> MATVEPETTPTPNPPTTEEEKTESNQEVANPEHYIKHPLQNRWALWFFKNDKSKTWQANLRLISKFDTVEDFWALYNHIQLSSNLMPGCDYSLFKDGI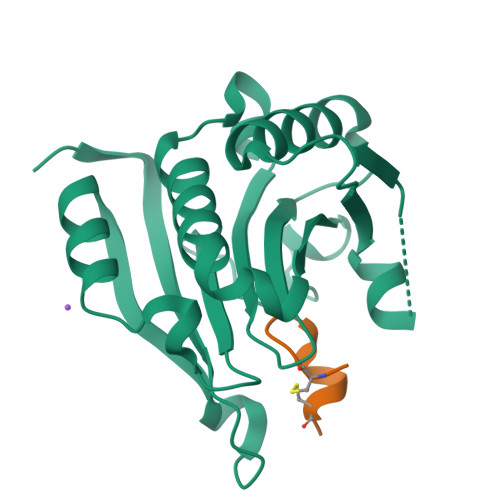EPMWEDEKNKRGGRWLITLNKQQRRSDLDRFWLETLLCLIGESFDDYSDDVCGAVVNVRAKGDKIAIWTTECENREAVTHIGRVYKERLGLPPKIVIGYQSHADTATKSGSTTKNRFVV;> ACEMGFFQDCGX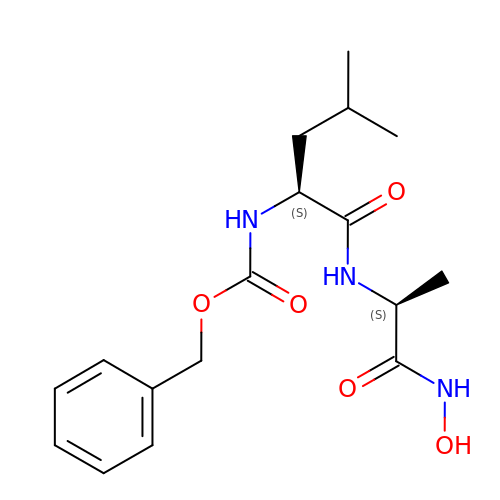N-[(benzyloxy)carbonyl]-L-leucyl-N-hydroxy-L-alaninamide | C17 H25 N3 O5 | GFVPLCZPHFWQIY-JSGCOSHPSA-N> MTARGLALGLLLLLLCPAQVFSQSCVWYGECGIAYGDKRYNCEYSGPPKPLPKDGYDLVQELCPGFFFGNVSLCCDVRQLQTLKDNLQLPLQFLSRCPSCFYNLLNLFCELTCSPRQSQFLNVTATEDYVDPVTNQTKTNVKELQYYVGQSFANAMYNACRDVEAPSSNDKALGLLCGKDADACNATNWIEYMFNKDNGQAPFTITPVFSDFPVHGMEPMNNATKGCDESVDEVTAPCSCQDCSIVCGPKPQPPPPPAPWTILGLDAMYVIMWITYMAFLLVFF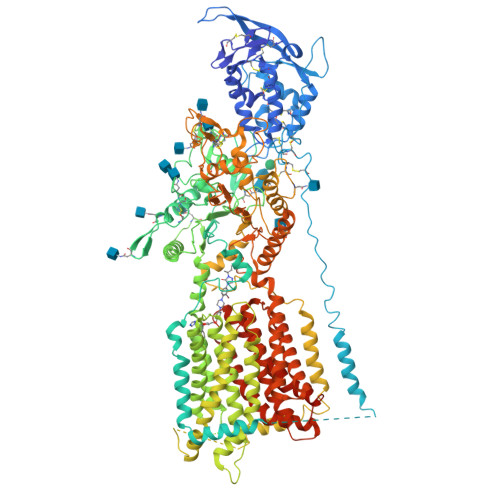GAFFAVWCYRKRYFVSEYTPIDSNIAFSVNASDKGEASCCDPVSAAFEGCLRRLFTRWGSFCVRNPGCVIFFSLVFITACSSGLVFVRVTTNPVDLWSAPSSQARLEKEYFDQHFGPFFRTEQLIIRAPLTDKHIYQPYPSGADVPFGPPLDIQILHQVLDLQIAIENITASYDNETVTLQDICLAPLSPYNTNCTILSVLNYFQNSHSVLDHKKGDDFFVYADYHTHFLYCVRAPASLNDTSLLHDPCLGTFGGPVFPWLVLGGYDDQNYNNATALVITFPVNNYYNDTEKLQRAQAWEKEFINFVKNYKNPNLTISFTAERSIEDELNRESDSDVFTVVISYAIMFLYISLALGHMKSCRRLLVDSKVSLGIAGILIVLSSVACSLGVFSYIGLPLTLIVIEVIPFLVLAVGVDNIFILVQAYQRDERLQGETLDQQLGRVLGEVAPSMFLSSFSETVAFFLGALSVMPAVHTFSLFAGLAVFIDFLLQITCFVSLLGLDIKRQEKNRLDIFCCVRGAEDGTSVQASESCLFRFFKNSYSPLLLKDWMRPIVIAIFVGVLSFSIAVLNKVDIGLDQSLSMPDDSYMVDYFKSISQYLHAGPPVYFVLEEGHDYTSSKGQNMVCGGMGCNNDSLVQQIFNAAQLDNYTRIGFAPSSWIDDYFDWVKPQSSCCRVDNITDQFCNASVVDPACVRCRPLTPEGKQRPQGGDFMRFLPMFLSDNPNPKCGKGGHAAYSSAVNILLGHGTRVGATYFMTYHTVLQTSADFIDALKKARLIASNVTETMGINGSAYRVFPYSVFYVFYEQYLTIIDDTIFNLGVSLGAIFLVTMVLLGCELWSAVIMCATIAMVLVNMFGVMWLWGISLNAVSLVNLVMSCGISVEFCSHITRAFTVSMKGSRVERAEEALAHMGSSVFSGITLTKFGGIVVLAFAKSQIFQIFYFRMYLAMVLLGATHGLIFLPVLLSYIGPSVNKAKSCATEERYKGTERERLLNFWSHPQFEK> GHMRRELAIEFSRVTESAALAGYKWLGRGDKNTADGAAVNAMRIMLNQVNIDGTIVIGEGEIAEAPMLYIGEKVGTGRGDAVDIAVDPIEGTRMTAMGQANALAVLAVGDKGCFLNAPDMYMEKLIVGPGAKGTIDLNLPLADNLRNVAAALGKPLSELTVTILAKPRHDAVIAEMQQLGVRVFAIPDGDVAASILTCMPDSEVDVLYGIGGAPEGVVSAAVIRALDGDMNGRLLARHDVKGDNEENRRIGEQELARCKAMGIEAGKVLRLGDMARSDNVIFSATGITKGD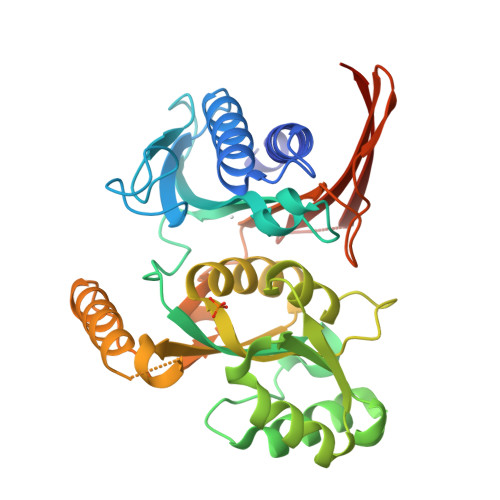LLEGISRKGNIATTETLLIRGKSRTIRRIQSIHYLDRKDPEMQVHIL(1R,4S,5S,6R)-4-(cyclohexylamino)-5,6-dihydroxy-2-(hydroxymethyl)cyclohex-2-en-1-yl alpha-D-glucopyranoside | C19 H33 N 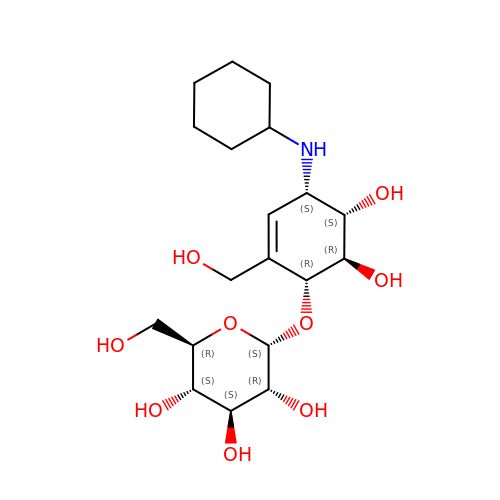O9 | YAIDDCWZVAZCDT-DXAFFUQDSA-N>[2x]SRFADAVLDQYIGSIHSLCKDQHGCRFL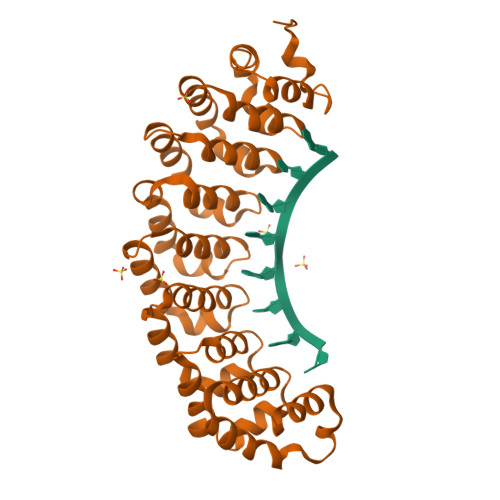QKQLDILGSKAADAIFEETKDYTVELMTDSFGNYLIQKLLEEVTTEQRIVLTKISSPHFVEISLNPHGCRALQKLIECIKTDEEAQIVVDSLRPYTVQLSKDLNGNHVIQKCLQRLKPENFQFIFDAISDSCIDIATHRHGCRVLQRCLDHGTTEQCDNLCDKLLALVDKLTLDPFGNYVVQYIITKEAEKNKYDYTHKIVHLLKPRAIELSIHKFGSNVIEKILKTAIVSEPMILEILNNGGETGIQSLLNDSYGNYVLQTALDISHKQNDYLYKRLSEIVAPLLVGPIRNTPHGKRIIGMLHLDS> MTLEKFVDALPIPDTLKPVQQSKEKTYYEVTMEECTHQLHRDLPPTRLWGYNGLFPGPTIEVKRNENVYVKWMNNLPSTHFLPIDHTIHHSDSQHEEPEVKTVVHLHGGVTPDDSDGYPEAWFSKDFEQTGPYFKREVYHYPNQQRGAILWYHDHAMALTRLNVYAGLVGAYIIHDPKEKRLKLPSDEYDVPLLITDRTINEDGSLFYPSAPENPSPSLPNPSIVPAFCGETILVNGKVWPYLEVEPRKYRFRVINASNTRTYNLSLDNGGDFIQIGSDGGLLPRSVKLNSFSLAPAERYDIIIDFTAYEGESIILANSAGCGGDVNPETDANIMQFRVTKPLAQKDESRKPKYLASYPSVQHERIQNIRTLKLAGTQDEYGRPVLLLNNKRWHDPVTETPKVGTTEIWSIINPTRGTHPIHLHLVSFRVLDRRPFDIARYQESGELSYTGPAVP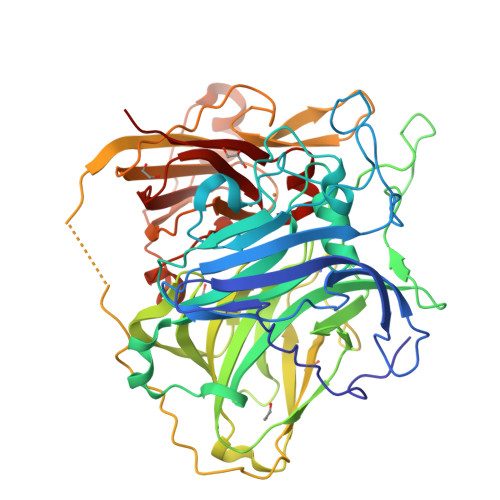PPPSEKGWKDTIQAHAGEVLRIAATFGPYSGRYVWHCCILEHEDYDMMRPMDITDPHK N-oxo-2-(phenylsulfonylamino)ethanamide 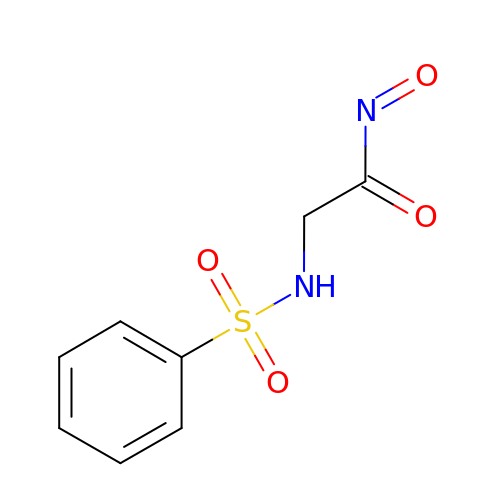| C8 H8 N2 O4 S | LBEMJFIVKDOIBO-UHFFFAOYSA-N R,3-HYDROXYBUTAN-2-ONE | C4 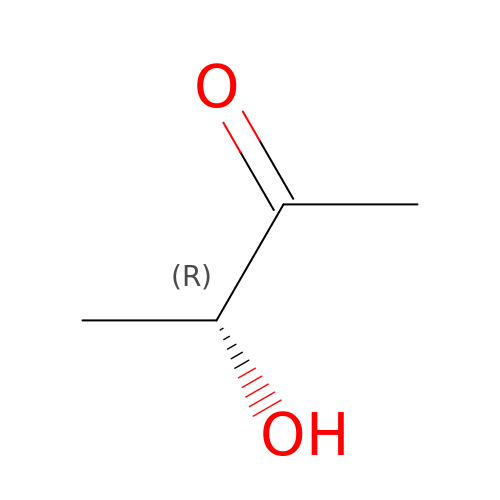H8 O2 | ROWKJAVDOGWPAT-GSVOUGTGSA-N>TPFKIAMVGRYSNEKNQSVLIKAVALSKYKQDIVLLLKGKGPDEKKIKLLAQKLGVKAEFGFVNSNELLEILKTCTLYVHAANVESEAIACLEAISVGIVPVIANSPLSATRQFALDERSLFEPNNAKDLSAKIDWWLENKLERE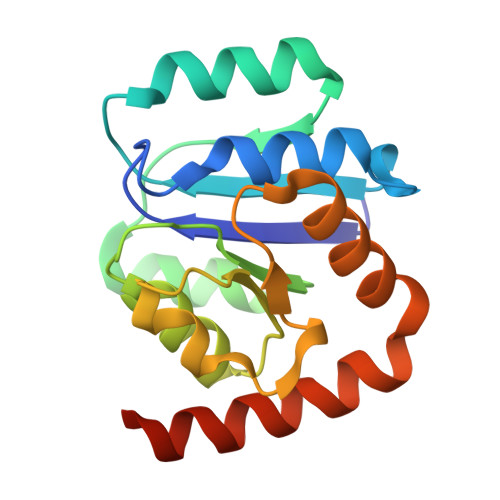RMQNEYAKSALNYTLENSVIQ[2x]> MSTRKIFDSEEQSFIRLVDKFYLGLSLTKLCAQSCNLLRNDISGSALTQK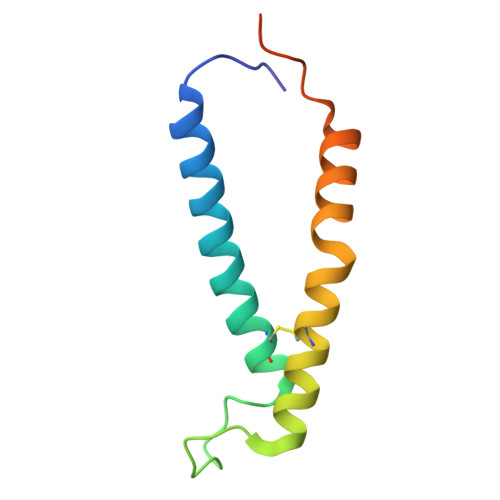EKDCLSICYNNIEKTQSAFYAKVKTTMNLPAVEDDGEEGGDDE>[4x]DSIMKILLIGDSGVGKSCLLVR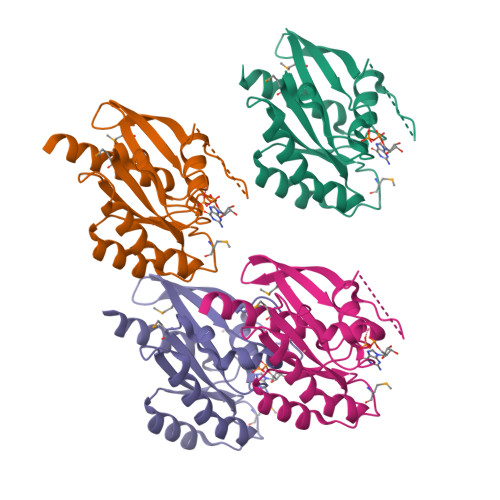FVEDKFNPSFITTIGIDFKIKTVDINGKKVKLQIWDTAGQERFRTITTAYYRGAMGIILVYDITDERTFTNIKQWFKTVNEHANDEAQLLLVGNKSDMETRVVTADQGEALAKELGIPFIESSAKNDDNVNEIFFTLAKLIQEKIDSN> MPAAAALSDDDRLVVAHCAALSFPPASQPPPPPTTSSSSSGAGAGASFQVHHASHPYPCAAFAFPPSWSAAPGWAAAGRAAFGDAEV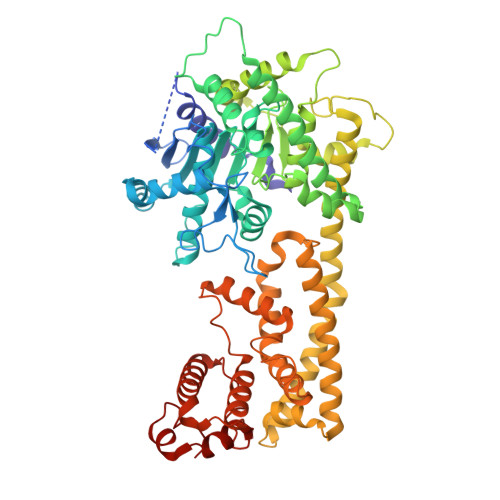DPSLFPSLRSVGSGVPARANAAFLASFGALLDGSPLQSEVSRAVAEEKRIVFTGHSSGGSIATLAAIWFLETCTRRGSVNQAHPFCVTFGAPLVGDNTFNNAVRREGWSQCILNFVVPVDIIPRIPLTPLASATEGIQAVLDWLSPQTPNFSPSGMPLIISQFYENLLRSTLSIASYEACSFMGCTSSILGTLTSFIELSPYRPCGTYLFLTSSEQLAVLTNSDAVLQLLFYCLQLDPQQQLRDAAERSLSAHWQYEPIKQSMMQEIVCVDYLGVVSSTLPGRQMSSTIVGGLELSKEAMLSLSAAGQWEKQRETNQAKIDGASCTKIREALKSLNEYKRTCELHEVSYYDSFKLQREVHDFNANVSRLELAGLWDEIVEMLRRRELPDGFESRQDWVNLGTLYRRLVEPLDIANYYRHSKNEDTGSYLSKGRPRRYKYTQEWHEQSQRISFGSSLESCFWAMAEELQAEIANGKTFEDVRDRVVKLESDAHGWSMSGSLGKDIFLSRSSFVIWWKTLPENHRSASCIAKLVPW(4S)-4-AMINO-5-[({3-HYDROXY-2-METHYL-5-[(PHOSPHONOOXY)METHYL]PYRIDIN-4-YL}METHYL)AMINO]PENTANOIC 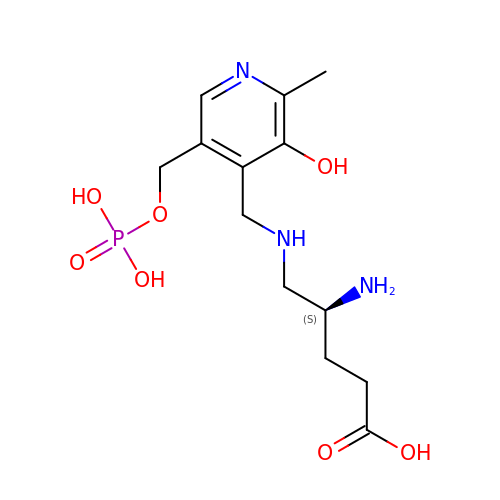ACID | C13 H22 N3 O7 P | DSCJVPXIMLLBAH-JTQLQIEISA-N> SLTERHKILHR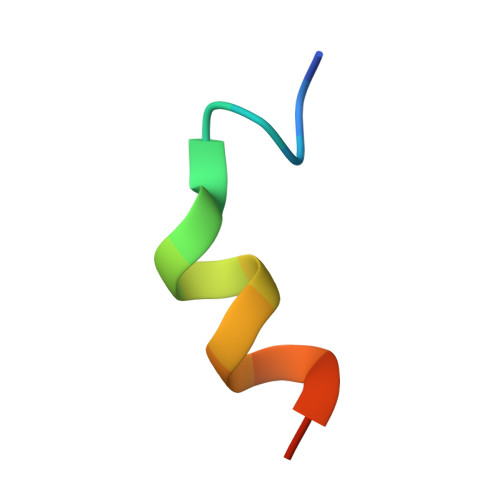LLQEGS>MADSELQLVEQRIRSFPDFPTPGVVFRDISPVLKDPASFRAAIGLLARHLKATHGGRIDYIAGLDSRGFLFGPSLAQELGLGCVLIRKRGKLPGPTLWASYSLEYGKAELEIQKDALEPGQRVVVVDDLLATGGTMNAACELLG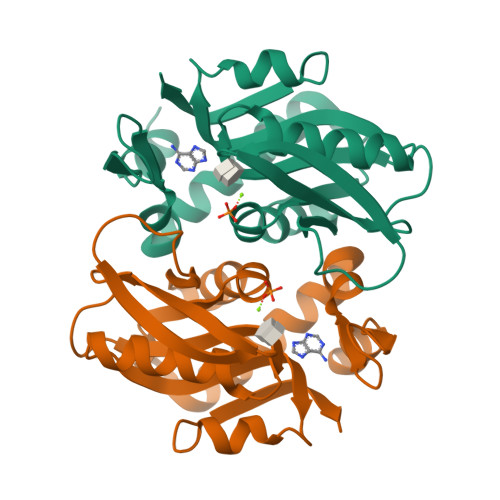RLQAEVLECVSLVELTSLKGREKLAPVPFFSLLQYE[2x]> KKGSVVIVGRINLSGDTAYAQQTRGEEGCQETSQTGRDKNQVEGEVQIVSTATQTFLATSINGVLWTVYHGAGTRTIASPKGPVTQMYTNVDKDLVGWQAP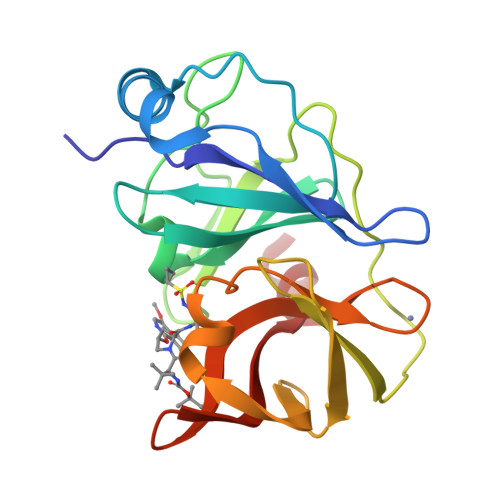QGSRSLTPCTCGSSDLYLVTRHADVIPVRRRGDSTGSLLSPRPLSYLKGSSGGPLLCPAGHAVGIFRAAVCTRGVAKAVQFIPVESLETTM>MTGSEIFLASKRAAITYDTDPATGEPRAWLAPGGTGNVVAEQAGVLNISWIASADSEDDRRASALNPDGVTMELHSGREILVRLIRHDPAVFRNVQNFMTANLMWAANNYGWDRWTQPSFGSDAREGWADFGRFTRDFADAILKSSAQSADPVYLVHDYQLVGVPALLREQRPDAPILLFVHIPWPSADYWRILPKEIRTGILHGMLPATTIGFFADRWCRNFLESVADLLPDARIDREAMTVEWRGHRTRLRTMPLGYSPLTLDGRNPQLPEGIEEWADGHRLVVHSGRTDPIKNAERAVRAFVLAARGGGLEKTRMLVRMNPNRLYVPANADYVHRVETAVAEANAELGSDTVRIDNDNDVNHTIACFRRADLLIFNS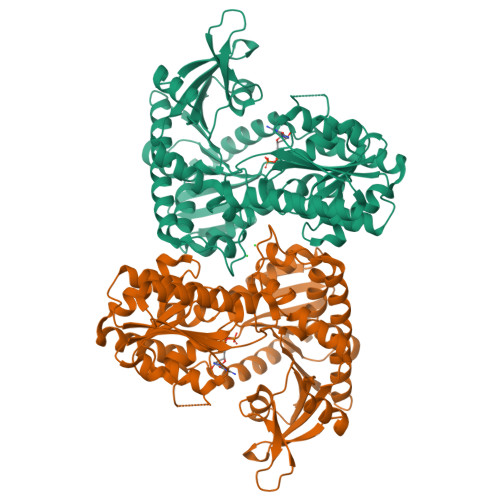TVDGQNLSTFEAPLVNERDADVILSETCGAAEVLGEYCRSVNPFDLVEQAEAISAALAAGPRQRAEAAARRRDAARPWTLEAWVQAQLDGLAADHAARTATAERFDTAPAVSTRADL[2x]The CysN polypeptide also contains a C-terminal APS (adenosine-5’-phosphosulfate) kinase domain (CysC), which exists as a separate enzyme in other bacteria and plants. Alternatively, APS can be phosphorylated at the 3′-position by APS kinase (CysC) to generate 3′-phosphoadenosine 5′-phosphosulfate (PAPS), a substrate for sulfotransferases that catalyze the transfer of the sulfate group onto a variety of metabolites. The structure of CysC is characterized by the canonical α/β-purine nucleotide binding fold, consisting of a five-stranded parallel β-sheet which is flanked on both sides by two α-helices. Structural features typical of APS kinases of this fold family, including the P-loop required for ATP binding (residues 452–458 in CysC), the conserved LDGD motif (residues 477–480) and the lid region (residues 552–581) above the P-loop which closes upon substrate binding, are also found in CysC.

The ADP complex crystallized in space group P21 with two molecules in the asymmetric unit. The asymmetric unit of the crystals of the CysC•ADP binary complex contains two subunits, which are related by a two-fold molecular symmetry axis. Manual inspection and analysis by the PISA server suggests a dimeric quaternary structure with a buried surface area of 3300 Å2, with the dominant part of the interface formed by interactions of residues from helices α2 and α3 with their symmetry mates. The ADP binding site in CysC is located in a crevice formed by the loop between β1 and α1 (residues 449–456), the loop 551–562 including helix α5 and the loop region 593–599. In each of the subunits the bound nucleotide was modeled in two different conformations that accounted best for the electron density map. The differences between both conformations are small; the adenine rings are slightly shifted with respect to each other due to a rotation of the glycosidic bond. ADP is bound to CysC in the anti conformation, similar to ADP binding in APS kinase from P. chrysogenum, but different from the situation in human PAPSS1 where both the syn and anti conformation were observed. The adenine ring of ADP is sandwiched between the guanidinium group of Arg559 and the side chain of Ile599. The NH2 group of adenine forms hydrogen bonds to the backbone carbonyl group of Arg597 and the side chain of Gln602. The diphosphate group is tightly anchored to the protein via the conserved P-loop at the N-terminus of helix α1 and the β phosphate interacts with main chain nitrogen atoms of residues 453–458.

>[2x]SPPRGKTVWFTGLSGSGKSSVAMLVERKLLEKGISAYVLDGDNLRHGLNADLGFSMADRAENLRRLSHVATLLADCGHLVLVPAISPLAEHRALARKVHADAGIDFFEVFCDTPLQDCERRDPKGLYAKARAGEITHFTGIDSPYQRPKNPDLRLTPDRSIDEQAQEVIDLLES>KADNSSVEKLVVQVQQLDPVKGNKDVGTVEITESAYGLVFTPHLHGLAQGLHGFHIHQNPSCEPKEKDGKLVAGLGAGGHWDPKETKQHGYPWSDNAHLGDLPALFVEHDGSATNPVLAPRLKKLDEVKGHSLMIHE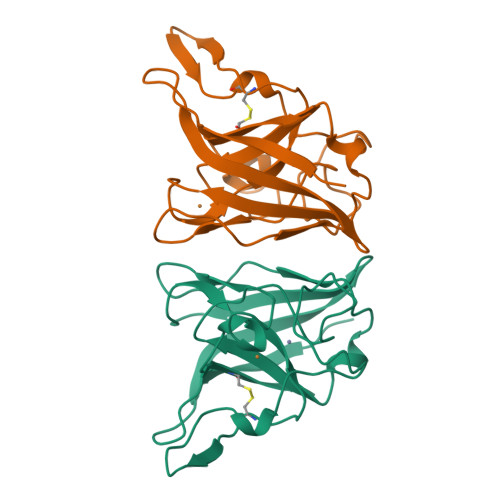GGDNHSDHPAPLGGGGPRMACGVIK[2x]>MKTSDANETEDHLESLICKVGEKSACSLESNLEGLAGVLEADLPNYKSKILRLLCTVARLLPEKLTIYTTLVGLLNARNYNFGGEFVEAMIRQLKESLKANNYNEAVYLVRFLSDLVNCHVIAAPSMVAMFENFVSVTQEEDVPQVRRDWYVYAFLSSLPWVGKELYEKKDAEMDRIFANTESYLKRRQKTHVPMLQVWTADKPHPQEEYLDCLWAQIQKLKKDRWQERHILRPYLAFDSILCEALQHNLPPFTPPPHTEDSVYPMPRVIFRMFDYTDDPEGPVMPGSHSVERFVIEENLHCIIKSHWKERKTCAAQLVSYPGKNKIPLNYHIVEVIFAELFQLPAPPHIDVMYTTLLIELCKLQPGSLPQVLAQATEMLYMRLDTMNTTCVDRFINWFSHHLSNFQFRWSWEDWSDCLSQDPESPKPKFVREVLEKCMRLSYHQRILDIVPPTFSALCPANPTCIYKYGDESSNSLPGHSVALCLAVAFKSKATNDEIFSILKDVPNPNQDDDDDEGFSFNPLKIEVFVQTLLHLAAKSFSHSFSALAKFHEVFKTLAESDEGKLHVLRVMFEVWRNHPQMIAVLVDKMIRTQIVDCAAVANWIFSSELSRDFTRLFVWEILHSTIRKMNKHVLKIQKELEEAKEKLARQHKRRSDDD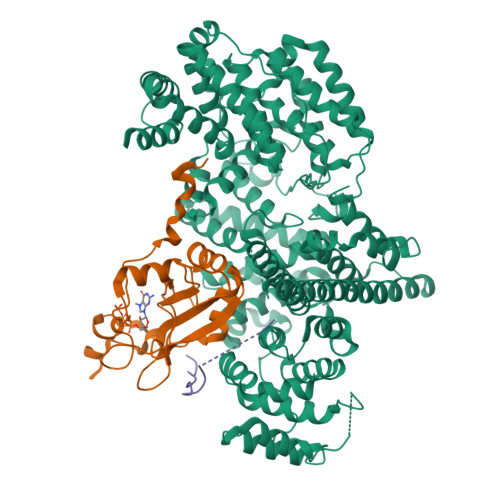DRSSDRKDGVLEEQIERLQEKVESAQSEQKNLFLVIFQRFIMILTEHLVRCETDGTSVLTPWYKNCIERLQQIFLQHHQIIQQYMVTLENLLFTAELDPHILAVFQQFCALQA[4x];>[4x]GAMSGGLLKALRSDSYVELSQYRDQHFRGDNEEQEKLLKKSCTLYVGNLSFYTTEEQIYELFSKSGDIKKIIMGLDKMKKTACGFCFVEYYSRADAENAMRYINGTRLDDRIIRTDWDAGFKEGRQYGRGRSGGQVRDEYRQDYDAGRGGYGKLAQNQ;>DKRTQIVYSDDVYKENLVDGF[3x]>GMTDQSVRIIEAALRLYMKKPPHEVSIEEIAREAKVSKSLIFYHFESKQKLLEEAVMHAFRKMMEEFNPRSVEEVVDYGIGFIAERREFIEFMMYALSQVRIEELERMFGEALEKVASLFEGCRHPRETAIALMAMLDGLS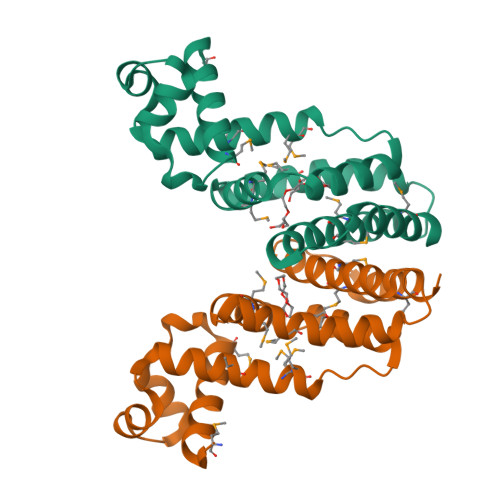IYSLYFDLGKLEKYREIAMEFVESRRVRA[2x]(S)-3-(3-(4-(2-GUANIDINOETHYL)PIPERIDIN-1-YL)-2-(NAPHTHALENE-2-SULFONAMIDO)-3-OXOPROPYL)BENZIMIDAMIDE | C28 H35 N7 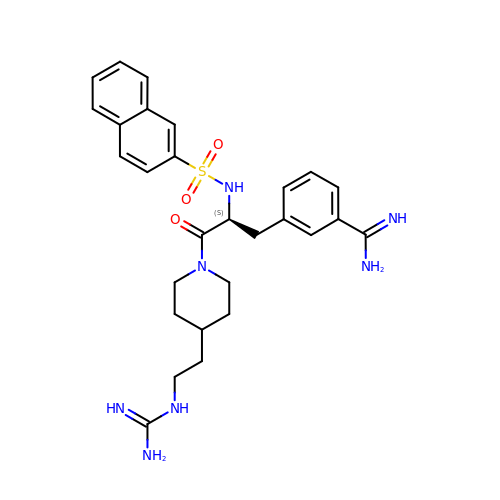O3 S | BKOKSJAQZJNVPN-VWLOTQADSA-N We use computational design coupled with experimental characterization to systematically investigate the design principles for macrocycle membrane permeability and oral bioavailability. We designed 184 6–12 residue macrocycles with a wide range of predicted structures containing noncanonical backbone modifications and experimentally determined structures of 35; 29 are very close to the computational models. With such control, we show that membrane permeability can be systematically achieved by ensuring all amide (NH) groups are engaged in internal hydrogen bonding interactions. The ability to robustly design membrane-permeable and orally bioavailable peptides with high structural accuracy should contribute to the next generation of designed macrocycle therapeutics.

We first tested the ability of our design pipeline to control both macrocycle structure and membrane permeability on 6–8 residue macrocycles spanning a diversity of structures and N-methylation patterns. For 6, 7, and 8 residue macrocycles, we selected 8, 5, and 19 designs (representing 6, 5, and 16 clusters), respectively, with fully satisfied backbone NH groups and funnel-like energy landscapes and spanning a diversity of sequences, structures, N-methylation patterns, and structural motifs (see Data S1 and S2 for sequences and design models). Selected macrocycles were chemically synthesized and purified using reverse-phase high-performance liquid chromatography (RP-HPLC). In some cases, two peaks were observed with the expected MW; in such cases we experimentally tested the two peaks separately and refer to these as p1 and p2 in the design names. To evaluate the accuracy of the design method, we determined X-ray crystal structures for two 7 residue designs and fifteen 8 residue designs. The structures for two 7 residue and twelve of the 8 residue macrocycles were very close to the computational design models (backbone atom RMSD < 1.2 Å). Having found that the macrocycles fold as designed, we next investigated their membrane permeabilities using transwell permeability assays. Eight 6-mers, five 7-mers, and sixteen 8-mers had apparent permeabilities (Papp) greater than 1 × 10−7 cm/s. Of these, eight 6-mers, five 7-mers, and ten 8-mers had Papp greater than 1 × 10−6 cm/s. In our 6–8 residue permeable designs, the number of N-methylated amino acids ranges between 0 and 3.

> LVPLLIPL>[12x]AETVSFS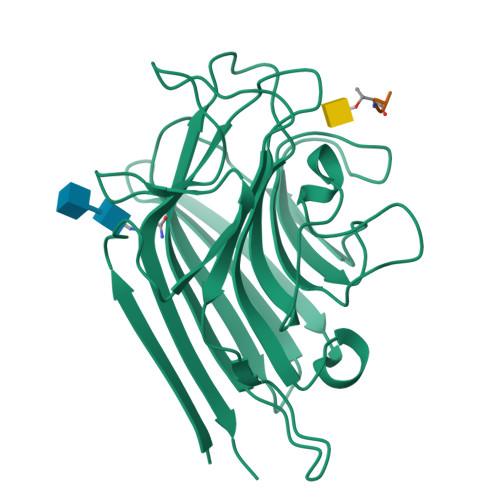WNKFVPKQPNMILQGDAIVTSSGKLQLNKVDENGTPKPSSLGRALYSTPIHIWDKETGSVASFAASFNFTFYAPDTKRLADGLAFFLAPIDTKPQTHAGYLGLFNENESGDQVVAVEFDTFRNSWDPPNPHIGINVNSIRSIKTTSWDLANNKVAKVLITYDASTSLLVASLVYPSQRTSNILSDVVDLKTSLPEWVRIGFSAATGLDIPGESHDVLSWSFASNLPHASSNIDPLDLTSFVLHEAI;>APDTR[12x]>MKNIHLIPYRVEQVTAAPPRIPEGVRMIQAPELWESAEHGKGNVVAVLDTGCQTDHPDLTARIAGGRNFTHDDGGDPERFEDYNGHGTHVAGTVAASLRDEEGVVGVAPLADLLVVKVLDKEGSGSYEGIIAGIHYAIDWRGPEGQKTTVISMSLGGPEDHPELYEAVKRAVDAGIPVICAAGNEGDDAHDTDEFAYPGAYGEVIQVGAVDFDRRIAPFSNTNNEIDLVAPGINIYSTYLEGKYASLSGTSMATPHVSGALALIRNISEREFDRELTEAELYAQLVRRT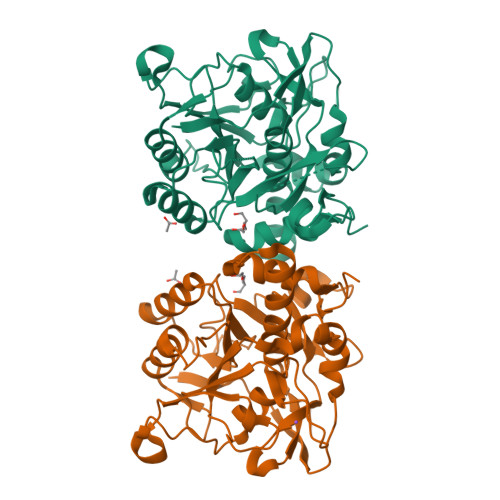IPLGYPKTAEGNGLLALDILNKFEQLFKILSNSYANGLDRA[2x]>[4x]MNDNVAWFKQAKYGMMIHWGLYSLLAGEYRGESSSAYAEWIQSKFQIPNAEYGNLATAFNPLYFDAKKIVALAKQCGMQYLVVTTKHHDGFAMYHSKVDAYNVYDATPFHRDIIGELAEACQKAGLKFGLYYSQDLDWHDPNGGGYKSNDVETAGTTWDNSWDFPDEDQKNFDLCFDNKILPQIKEIMSNYGDIATAWFDVPMTLSEAQSQTIYDTVRELQPNCLINSRLGNGKYDFVSLGDNEIPKNKE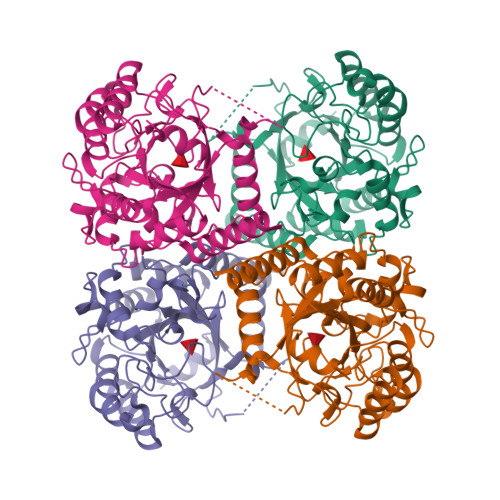DMNKTDVDYNEITGFKPSPLGLYETAGTINDSWGFSYHDQNWKTPRTLYRYKQHLNDFGINYLLNVGLDPLGRVPMMAEENLLAAKALEDEANRL> MASMTGGLEHPQFEKLEQKLISEEDLEDLAYPLLGTRIVLDEEKILKEGKYNLEDMYKMIDEYAKESGMIKINKETYHCKGDKY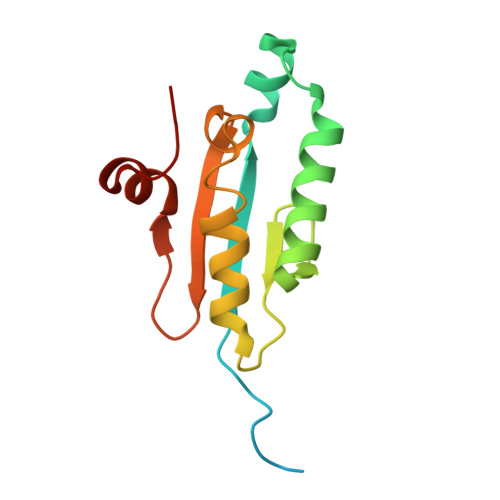DLGCMTLFIYKYLIDSEWFTKNAKEWIWISEKEGNSDLISASKAEGEGIWE> GMPGREILVLHVGQGGNQIGYNFWKTICEEHNIDIRSNQRKSVEEDKVDYKSVFLVEAPDGFHPRALFIDLEPLAVEFLVKEMKLGSFFSEDLMVLSYSGAHNVWSIGYQTGKKLIPVILEKIRDTMPETLQGFLIIHTLGGGTGSGFGSLLTETLKKEFPGKGVLNFSVLPSEVNDVTLAPYNTVLSLNHLSRFSDLVVLFDNTALIRIVKDQLNYPVIKQFSDLNFLIGRVMASITASLRFPGPLNMDLMEMAHNLVALPETKFIIPSVAPLTKEESEM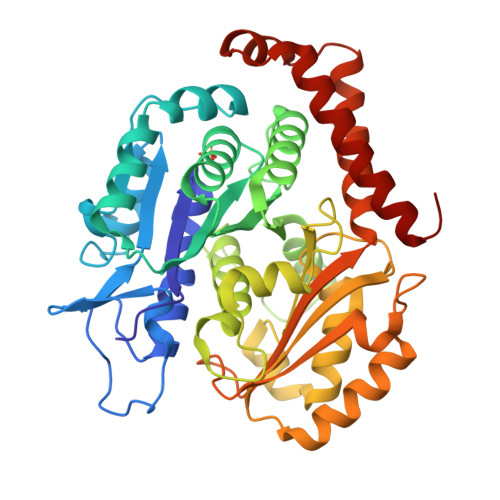STELDLVERCFDPTHYMVNCSGQGKTISSVLMFRGNIAIENAFSIMTDIKSNVAFAPGVHPDLGLKYGICESAPVDFDKEVTLLSNNTIISEVFNRVLERFDSLFNRDWYTSDYVNAGTSKSNLKEARDNFDRIIKIYKEIEGSQ> MSSKY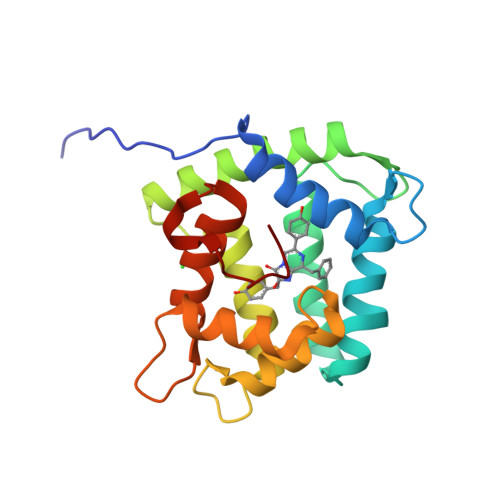AVKLKTDFDNPRWIKRHKHMFDFLDINGNGKITLDEIVSKASDDICAKLEATPEQTKRHQVCVEAFFRGCGMEYGKEIAFPQFLDGWKQLATSELKKWARNEPTLIREWGDAVFDIFDKDGSGTITLDEWKAYGKISGISPSQEDCEATFRHCDLDNSGDLDVDEMTRQHLGFWYTLDPEADGLYGNGVP> MSDLVLGLDIGIGSVGVGILNKVTGEIIHKNSRIFPAAQAENNLVRRTNRQGRRLTRRKKHRRVRLNRLFEESGLITDFTKISINLNPYQLRVKGLTDELSNEELFIALKNMVKHRGISYLDDASDDGNSSIGDYAQIVKENSKQLETKTPGQIQLERYQTYGQLRGDFTVEKDGKKHRLINVFPTSAYRSEALRILQTQQEFNPQITDEFINRYLEILTGKRKYYHGPGNEKSRTDYGRYRTSGETLDNIFGILIGKCTFYPDEFRAAKASYTAQEFNLLNDLNNLTVPTETKKLSKEQKNQIINYVKNEKAMGPAKLFKYIAKLLSCDVADIKGYRIDKSGKAEIHTFEAYRKMKTLETLDIEQMDRETLDKLAYVLTLNTEREGIQEALEHEFADGSFSQKQVDELVQFRKANSSIFGKGWHNFSVKLMMELIPELYETSEEQMTILTRLGKQKTTSSSNKTKYIDEKLLTEEIYNPVVAKSVRQAIKIVNAAIKEYGDFDNIVIEMARETNEDDEKKAIQKIQKANKDEKDAAMLKAANQYNGKAELPHSVFHGHKQLATKIRLWHQQGERCLYTGKTISIHDLINNSNQFEVDHILPLSITFDDSLANKVLVYATANQEKGQRTPYQALDSMDDAWSFRELKAFVRESKTLSNKKKEYLLTEEDISKFDVRKKFIERNLVDTRYASRVVLNALQEHFRAHKIDTKVSVVRGQFTSQLRRHWGIEKTRDTYHHHA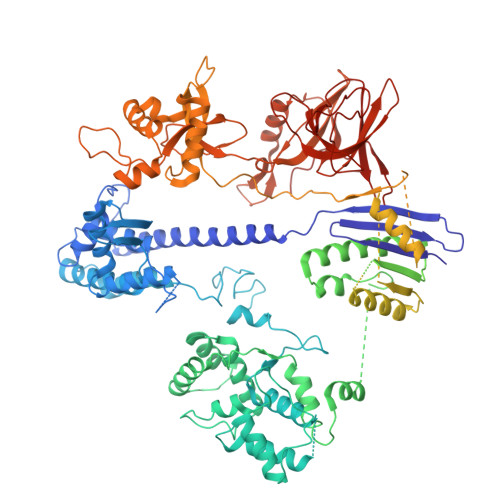VDALIIAASSQLNLWKKQKNTLVSYSEDQLLDIETGELISDDEYKESVFKAPYQHFVDTLKSKEFEDSILFSYQVDSKFNRKISDATIYATRQAKVGKDKADETYVLGKIKDIYTQDGYDAFMKIYKKDKSKFLMYRHDPQTFEKVIEPILENYPNKQINEKGKEVPCNPFLKYKEEHGYIRKYSKKGNGPEIKSLKYYDSKLGNHIDITPKDSNNKVVLQSVSPWRADVYFNKTTGKYEILGLKYADLQFEKGTGTYKISQEKYNDIKKKEGVDSDSEFKFTLYKNDLLLVKDTETKEQQLFRFLSRTMPKQKHYVELKPYDKQKFEGGEALIKVLGNVANSGQCKKGLGKSNISIYKVRTDVLGNQHIIKNEGDKPKLDF> MAGPIIAGKSESSELPRVEDRATFIYIEHAKINRVDSAVTVAEAKGVVRIPAAMIGVLLLGPGTDISH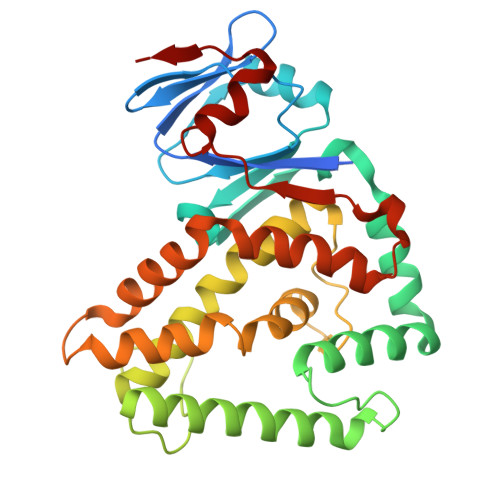RAVELLGDTGTALVWVGEQGVRYYASGRALARSTRFLVKQAELVTNERSRLRVARRMYQMRFPTEDVSKLTMQQLRSHEGARVRRKYRELSKKYNVPWKKRVYNPDDFAGGDPINQALSAAHVALYGLVHSVVAALGLSPGLGFVHTGHDRSFIYDVADLYKAEITVPIAFAVAAEAEEGQDIGQLARLRTRDAFVDGKILKRMVKDLQTLLEIPEEGQIEAEPLSLWDDKEKLVPYGVNYSE>MPVLENRAAQGDITAPGGARRLTGDQTAALRDSLSDKPAKNIILLIGDGMGDSEITAARNYAEGAGGFFKGIDALPLTGQYTHYALNKKTGKPDYVTDSAASATAWSTGVKTYNGALGVDIHEKDHPTILEMAKAAGLATGNVSTAELQHATPAALVAHVTSRKCYGPSATSEKCPGNALEKGGKGSITEQLLNARADVTLGGGAKTFAETATAGEWQGKTLREQAQARGYQLVSDAASLNSVTEANQQKPLLGLFADGNMPVRWLGPKATYHGNIDKPAVTCTPNPQRNDSVPTLAQMTDKAIELLSKNEKGFFLQVEGASIDHQDHAANPCGQIGETVD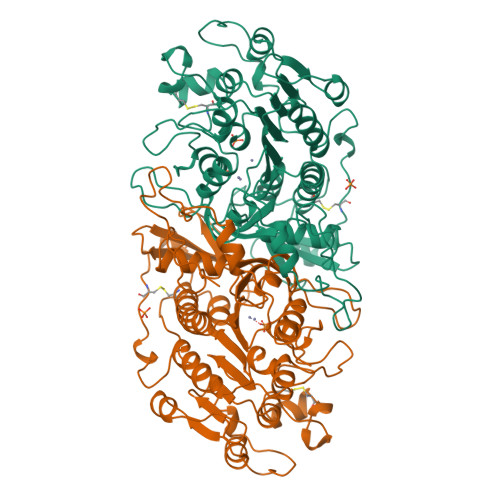LDEAVQRALEFAKKEGNTLVIVTADHAHASQIVAPDTKAPGLTQALNTKDGAVMVMSYGNSEEDSQEHTGSQLRIAAYGPHAANVVGLTDQTDLFYTMKAALGLK[2x]4-fluoro-5-hexyl-2-(2-methylphenoxy)phenol | C19 H23 F O2 | 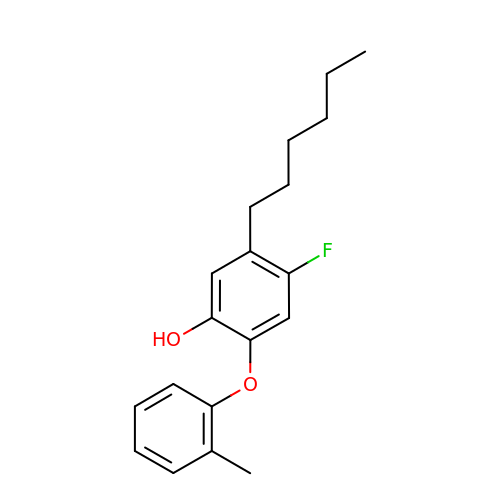GJZJMPMJSFDTJH-UHFFFAOYSA-N S-BENZYL 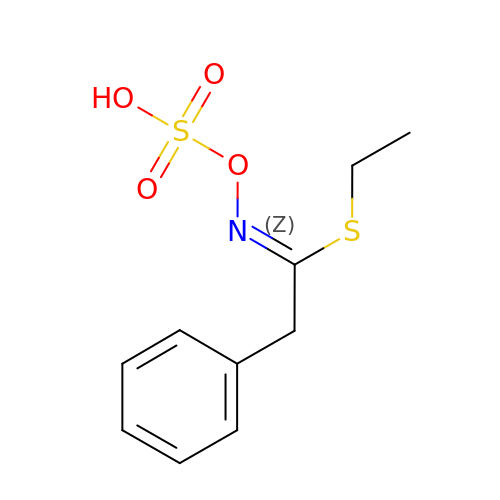PHENYLACETOTHIOHYDROXIMATE-O-SULFATE | C10 H13 N O4 S2 | VZFUNHITNWTQFU-KHPPLWFESA-N>[2x]CYCRIPACIAGERR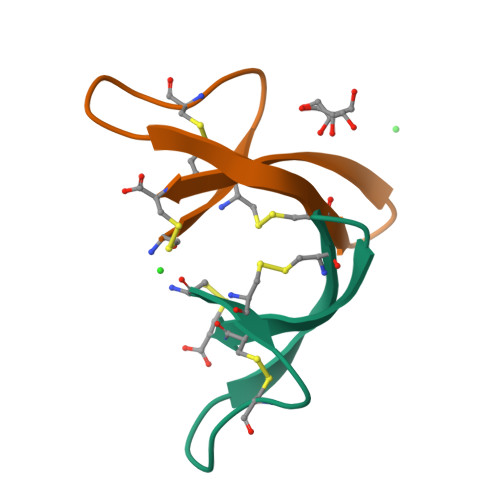YATCIYQGRLWAFCC>GSHMTPTPRPTDGVDIYFGMPGEISEHEGFLRAKMDLEERRMRQINEVMREWAMADNQSKNLPKADRQALNEHFQSILQTLEEQVSGERQRLVETHATRVIALINDQRRAALEGFLAALQADPPQAERVLLALRRYLRAEQKEQR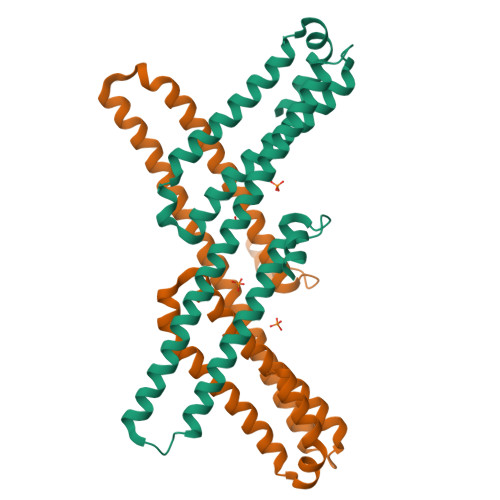HTLRHYQHVAAVDPEKAQQMRFQVHTHLQVIEERVNQSLGLLDQNPHLAQELRPQIQELLHSEHLGPSELEAPA[2x]> DKSYCGFIAIVGRPNVGKSTLLNKLLGQKISITSRKAQTTRHRIVGIHTEGAYQAIYVDTPGLHMEEKRAINRLMNKAASSSIGDVELVIFVVEGTRWTPDDEMVLNKLREGKAPVILAVNKVDNVQEKADLLPH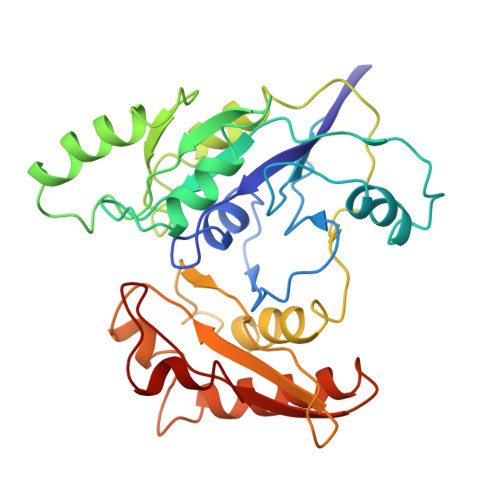LQFLASQMNFLDIVPISAETGLNVDTIAAIVRKHLPEATHHFPEDYITDRSQRFMASEIIREKLMRFLGAELPYSVTVEIERFVSNERGGYDINGLILVEREGQKKMVIGNKGAKIKTIGIEARKDMQEMFEAPVHLELWVKVKSGWADDERALRSL(2Z,5E)-6-[4-(4-fluorobenzoyl)-1H-pyrrol-2-yl]-2-hydroxy-4-oxohexa-2,5-dienoic acid | C17 H12 F N O5 | 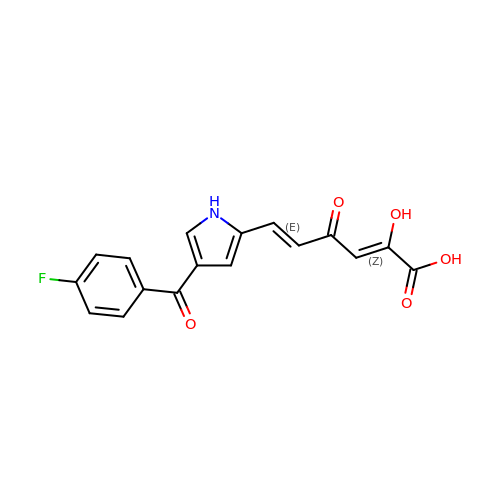XOINLIFLBUUBGT-RSIRFQHMSA-N>[6x]MATVLSPNQNNNSGSIPTGYSDLEFSLANGNWVKNLSLPTNANNSDKITIRSSAAYSSYLDTSNTNIPLEVLKINSGDVYQFIFNSSQNKWIAQLATVSPTTGSNYELIPLTTATMQKVLIQDDKWAQTIALPSDVRDGTTVQVVSTASVSSDIDKTNLLFPSSFTLKNGSEYWFKYYSALGKWVPEYIKPQKLNVQQIGTSLAAVNSPLTEIAFGDGNWVSNFTLPTTANDRDRIIIKSTATWSAKINNTNVNSQATLTLKTGDQYEFMYVSDKGYWQLISSPTKVIDSTATIPAILPNMTQPTLKVKLSTSNWQPTLQLPAQAQVGDKVVIVSNASADTYINAANGLSTAIKNGENRRFIYTAQGWTVDSYTIDMLLVSSPEVN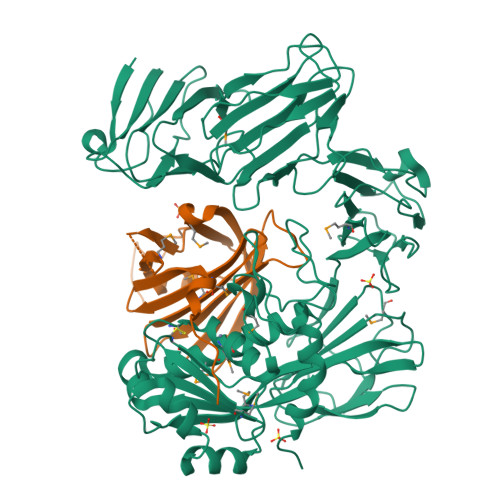SILGESAAKLRMIEGVNLTNLTAENSNARFYLRDVGYITYKIPAATLKEAISTGRDDTTVQNERKRILADGVYYQGNEPGDGGCGWAWINASAYNMIGANDIAGCSFAAMRHEVGHNLGLYHNGSTNIGSGFAHPLGSTAMGGNNINFYSSPYLYNPKYGVRLGEEGKIDAVSVINLNAQKISLYNHHHHHH;>[6x]MQSSSALTFSPESRQQSGAKMIESQNILNLSPSEKERLSQQQIVFNEVEKDQLHSKANFPLLKNAKGMVIKYDPKVIELKKVGDTVKFQMLEYGINRTGKIVEIEPVDQDIVRWTGRFDQGDPNQNFFTITQSQKDHYTIMQIFTEKGNYSAEIKDGVGLVQTMDEGVTDQELHHDHP> HHHHHHMVRAIDEDCSQYEPIPGSQKAALGYNILTQEDAQSVYDASYYGGQCETVYNGEWRELRYDSTCERLYYGDDEKYFRKPYNFLKYHFEALADTGISSEFYDNANDLLSKVKKDKSDSFGVTIGIGPAGSPLLVGVGVSHSQDTSFLNELNKYNEKKFIFTRIFTKVQTAHFK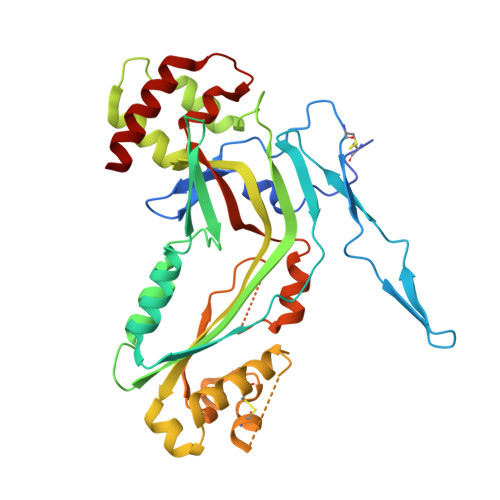MRKDDIMLDEGMLQSLMELPDQYNYGMYAKFINDYGTHYITSGSMGGIYEYILVIDKAKMESLGITSRDITTCFGGSLGIQYEDKINVGGGLSGDHCKKFGGGKTERARKAMAVEDIISRVRGGSSGWSGGLAQNRSTITYRSWGRSLKYNPVVIDFEMQPIHEVLRHTSLGPLEAKRQNLRRALDQYLM6-ethyl-5-{3-[3-(isoquinolin-5-yl)-5-methoxyphenyl]prop-1-yn-1-yl}pyrimidine-2,4-diamine 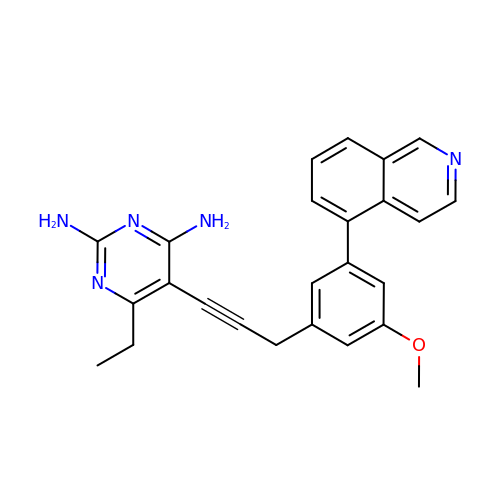| C25 H23 N5 O | IZQBFFXMDOOSIE-UHFFFAOYSA-N>[2x]MEKVPGEMEIERRERSEELSEAERKAVQAMWARLYANSEDVGVAILVRFFVNFPSAKQYFSQFKHMEDPLEMERSPQLRKHASRV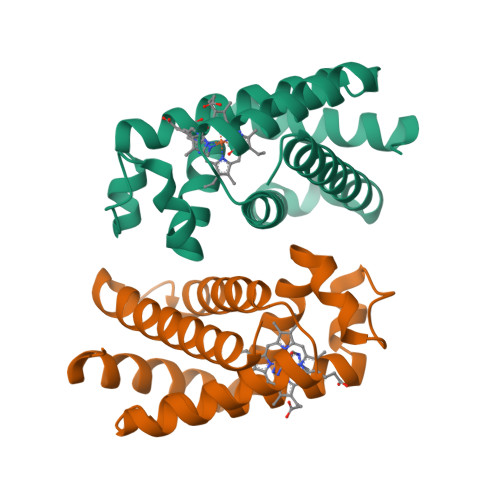MGALNTVVENLHDPDKVSSVLALVGKAHALKHKVEPVYFKILSGVILEVVAEEFASDFPPETQRAWAKLRGLIYSHVTAAYKEVGWVQQVPNATTPPATLPSSGP>[16x]SMGNPQLISAGAKFRAAVAAEQPLQVVGAITAYAAKMAEAVGFKAVYLSGGGVAANSLGIPDLGISTMDDVLVDANRITNATNLPLLVDIDTGWGGAFNIARTIRSFIKAGVGAVHLEDQVGQKRCGHRPGKECVPAGEMVDRIKAAVDARTDETFVIMAR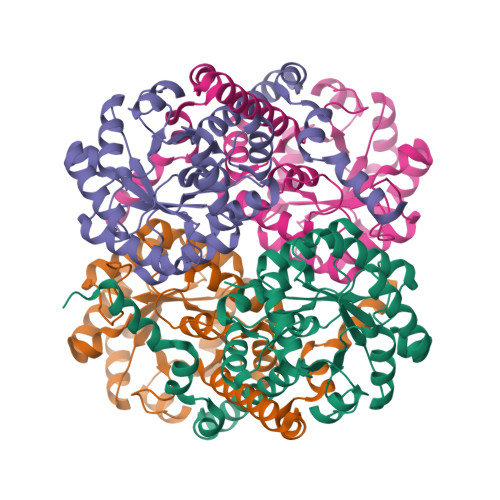TDAAAAEGIDAAIERAIAYVEAGADMIFPEAMKTLDDYRRFKEAVKVPILANLTEFGSTPLFTLDELKGANVDIALYCCGAYRAMNKAALNFYETVRRDGTQKAAVPTMQTRAQLYDYLGYYAYEEKLDQLFNQGRN> TQKPSLYRVLILNDDYTPAEFVVYVLERFFNKSREDATRIMLH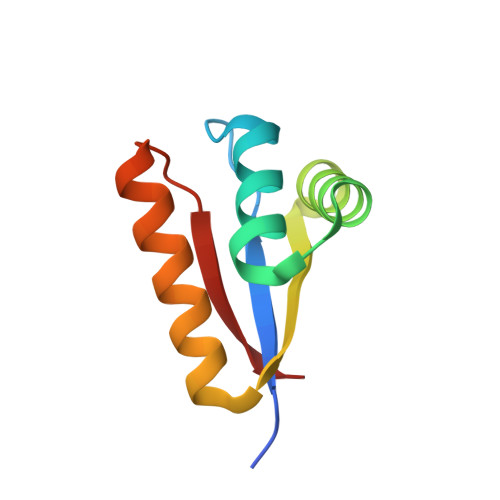VHQNGVGVCGVYTYEVAETKVAQVIDSARRHQHPLQCTMEKD> SYIKPLPSGDFIVKALTPVDAFNDFFGSEFSDEEFDTVGGLVMSAF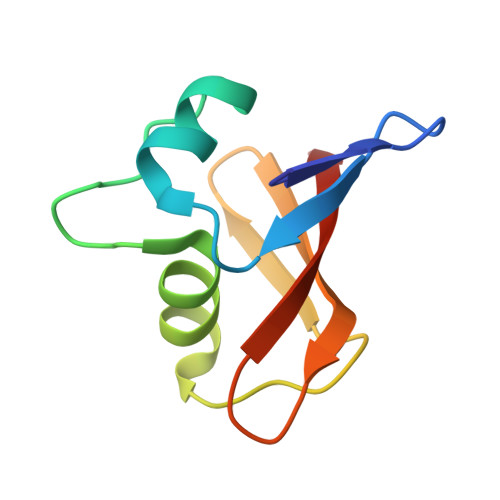GHLPKRNEVVELGEFRFRVLNADSRRVHLLRLSPLQN> GSHMSASAEPESDVKGRILDAAADAFMLRGFANTTIDDIADDVGATAGLIYYHFRSKFDIFLAVYEDGMRRVRERVEPYVGAPGTGRQRLVAMSVAHVENLMIDLGYHHVVHQGVRDQASTALKVRQRDALAALNELRRDYERMFHHVITE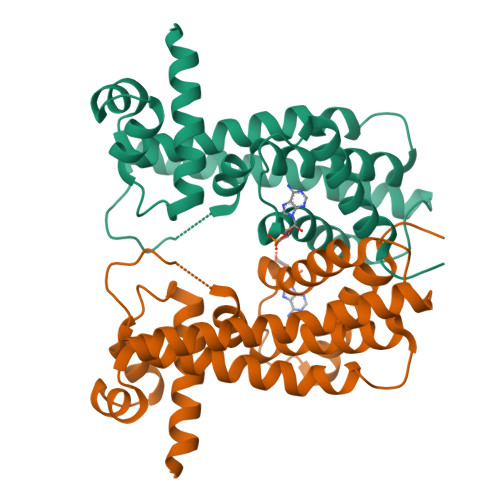GIADGSLRNVDDALATRTLLSNLNAVDVWYRKIEGQTEKEVHDLASQVVDLLIGGIGATAD> SLEAILPQLKCHFTWNLFREGSMSSHMEDRVCNQVEHLNSEEKATMYDLLAYIKHLDGESKAALECLGQAEDLRKSEHNDQSEIRRLVTWGNYAWIYYHMGRLSEAQAYVDKVRQVCQKFANPYSMECPELECEEGWTRLKCGRNERAKMCFEKALE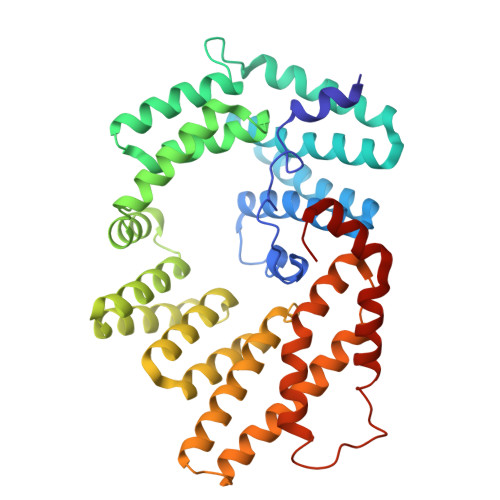EKPKDPECSSGMAIAMFRLEEKPEKQFSVDALKQAMELNPQNQYLKVLLALKLLRMGEEAEGERLIKDALGKAPNQTDVLQKAAQFYKKKGNLDRAIELLGKALRSTVNNSPLYSLVMCRYREILEQLQNKGDADSSERRQRMAELRRLTMEFMQKTLQRRRSPLNSYSDLIDFPEVERCYQMVISKESPDVEEEDLYERYCNLQEYHRKSEDLAALECLLQFPR>MAELAKSAVLVSSCTDDLLGDAKQVVVGPNQEDLHSAEAVLNRYSTVGFQASNLARAFSICEMMLTPQSPSPSLMPTEGDQASESPVMVQPTLFVGVTANLFGTGCREAIRFLCTECVPLPNGVEPATPLDDMAGISCDGTGALKPSPCDSRALIHVLVVSGGAMEHDIRRACESYKLSRDGAEEEGEQFHHPVERDRSRSKGTDCHFGNVRYNSSGVASRNLFSCVMRCLVKRLAEAQRKEKANREAAPIPEAYYDVCSWAITPSTLWYMAGLWMADIFTEALQETGEVTDEKVASEEGLKRAKSTVLYWAARNGVPIFSPSLTDGDIMEFILTAGDTGVPLLQLDLVADIHRLNRLAMRSRRTGMMILGGGVVKHHVCNANLMRNGADYAVFLNNAQEFDGSDAGARPGEAVSWGKLRLDSTAVKVYSEVTIVFPLIVVHVFVAWVRMMRSKGKENIRS[6x];>[6x]MSGVPFPSRVIGDLDYSNLLNIGQEEAIRCVLNAYPNIGLEATNLG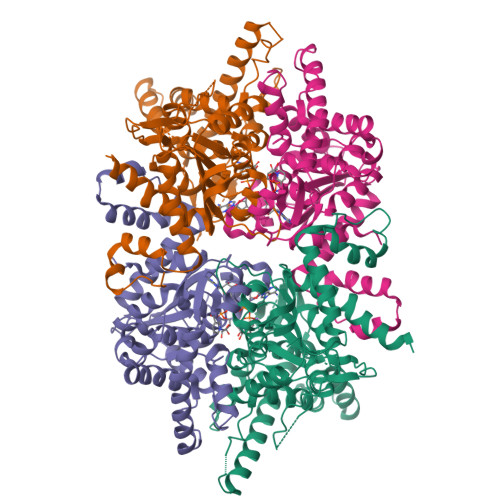RARRIVQRALNDNGMDGNKVMLAYTSNLISSGLRDTFACLARENRIGAVVTTAGGVEEDVIKCLGDTLVGDFALNDHALRNNGLNRVGNLLVPNDNYRNFEDFFVPLLRRLHEQQRDSRWTTKTTPSQIIAEIGAALESVRPNDCGSSLIYWCYRNDIPVFSPAFTDGSMGDMIYFYNYSRKGLVVDPVPDVRRLRQLGCKSTNVGRITCIVLGAGLPKHHLLRNVQADAVVYVTTGSDADGCESSCNVMADRANGLLSPNCDVVRVHGDATIISPLLLLRSSDGKEKVGVREDGN>[2x]LPTQPRDIENFNSTQKF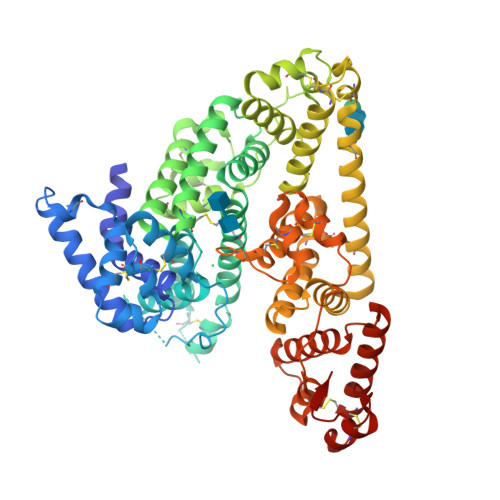IEDNIEYITIIAFAQYVQEATFEEMEKLVKDMVEYKDRCMADKTLPECSKLPNNVLQEKICAMEGLPQKHNFSHCCSKVDAQRRLCFFYNKKSDVGFLPPFPTLDPEEKCQAYESNRESLLNHFLYEVARRNPFVFAPTLLTVAVHFEEVAKSCCEEQNKVNCLQTRAIPVTQYLKAFSSYQKHVCGALLKFGTKVVHFIYIAILSQKFPKIEFKELISLVEDVSSNYDGCCEGDVVQCIRDTSKVMNHICSKQDSISSKIKECCEKKIPERGQCIINSNKDDRPKDLSLREGKFTDSENVCQERDADPDTFFAKFTFEYSRRHPDLSIPELLRIVQIYKDLLRNCCNTENPPGCYRYAEDKFNETTEKSLKMVQQECKHFQNLGKDGLKYHYLIRLTKIAPQLSTEELVSLGEKMVTAFTTCCTLSEEFACVDNLADLVFGELCGVNENRTINPAVDHCCKTNFAFRRPCFESLKADKTYVPPPFSQDLFTFHADMCQSQNEELQRKTDRFLVNLVKLKHELTDEELQSLFTNFANVVDKCCKAESPEVCFNEESPKIGNKGENLYFQ> MSICPHIQQVFQN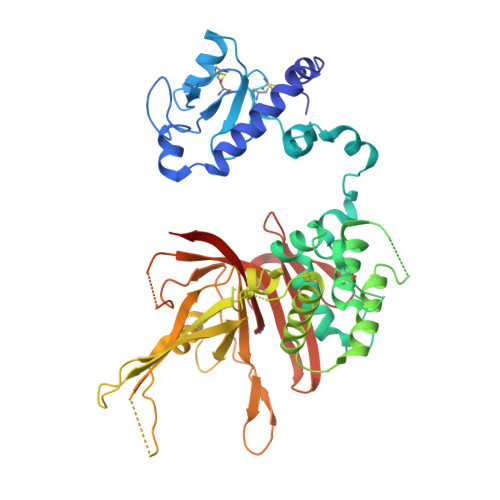EKSKDGVLKTCNAARYILNHSVPKEKFLNTMKCGTCHEINSGATFMCLQCGFCGCWNHSHFLSHSKQIGHIFGINSNNGLLFCFKCEDYIGNIDLINDAILAKYWDDVCTKTMVPSMERRDGLSGLINMGSTCFMSSILQCLIHNPYFIRHSMSQIHSNNCKVRSPDKCFSCALDKIVHELYGALNTKQASSSSTSTNRQTGFIYLLTCAWKINQNLAGYSQQDAHEFWQFIINQIHQSYVLDLPNAKEVSRANNKQCECIVHTVFEGSLESSIVCPGCQNNSKTTIDPFLDLSLDIKDKKKLYECLDSFHKKEQLKDFNYHCGECNSTQDAIKQLGIHKLPSVLVLQLKRFEHLLNGSNRKLDDFIEFPTYLNMKNYCSTKEKDKHSENGKVPDIIYELIGIVSHKGTVNEGHYIAFCKISGGQWFKFNDSMVSSISQEEVLKEQAYLLFYTIRQVN> MSDKVDIYSDRGKLLASDVDIMDLAPTRNRAIRTIIHDTKRTAAVNLGGIEKALANGRIGKVKKIPGKEMKLDIVANAERLAERVKELVQVNEGDDTTVEVLAGGKFLKVQVPSARLESGAEYVSSITASAAAITQAIIELFDVGIFDACMVKAAVWGDYPQTIGLNGGNVSSILEIPQKDEGLGFTLRNIMANHIAAITQRNAMNAAALSSILEQCGEFEMGNAIGMFERHQLLGLAYQGLNANNIVYETVKEQGKSGTIGTVVHSIVERALEDGVISVDKVAPSGYKFYKANDVMLWNAYAAAGSLAATMVNCGAARAAQCVSSTLLYFND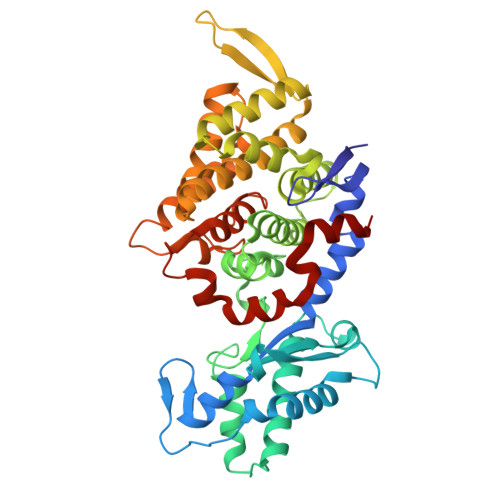LLEKETGLPGCDYGKVQGTAVGFSFFSHSIYGGGGPGVFNGNHIVTRHSRGFAIPCVAAAVALDAGTQMFSPEMTSAVVGTVYGSIPEFREPIKTVAASL(E)-2-METHYL-3-PHOSPHONOACRYLATE 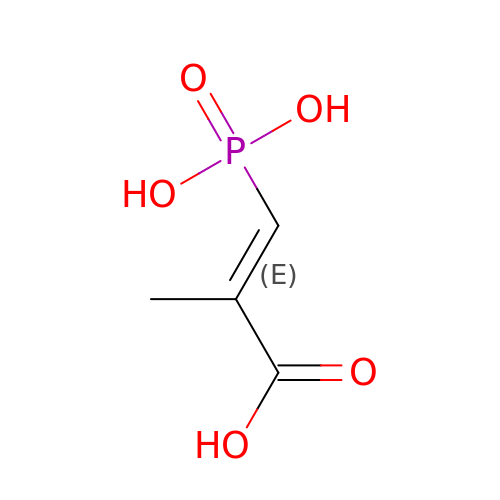| C4 H7 O5 P | XGDAHZFVQMTYCT-NSCUHMNNSA-N>[4x]NNELSPVALRQMSCAAGTTQTACTDDNALAYYNNSKGGRFVLALLSDHQDLKWARF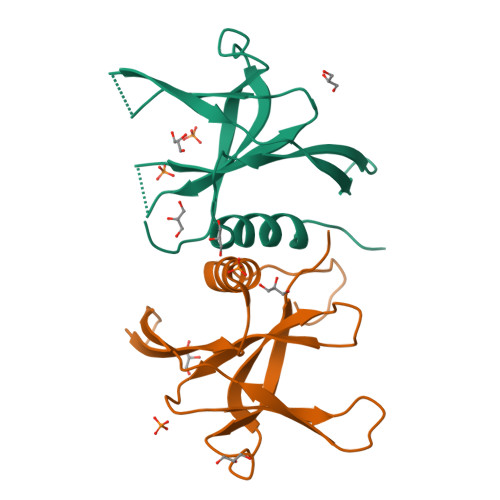PKSDGTGTIYTELEPPCRFVTDTPKGPKVKYLYFIKGLNNLNRGMVLESLAATVRLQLEHHHHHH>[2x]TPEMPVLENRAAQGDI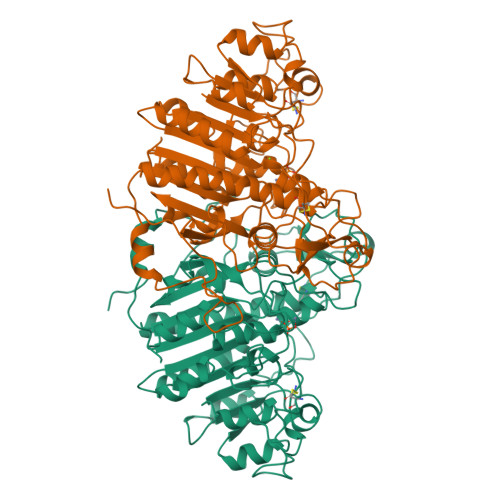TAPGGARRLTGDQTAALRDSLSDKPAKNIILLIGDGMGDSEITAARNYAEGAGGFFKGIDALPLTGQYTHYALNKKTGKPDYVTDAAASATAWSTGVKTYNGALGVDIHEKDHPTILEMAKAAGLATGNVSTAELQDATPAALVAHVTSRKCYGPSATSEKCPGNALEKGGKGSITEQLLNARADVTLGGGAKTFAETATAGEWQGKTLREQAQARGYQLVSDAASLNSVTEANQQKPLLGLFADGNMPVRWLGPKATYHGNIDKPAVTCTPNPQRNDSVPTLAQMTDKAIELLSKNEKGFFLQVEGASIDKQDHAANPCGQIGETVDLDEAVQRALEFAKKEGNTLVIVTADHAHASQIVAPDTKAPGLTQALNTKDGAVMVMSYGNSEEDSQEHTGSQLRIAAYGPHAANVVGLTDQTDLFYTMKAALGLK The mammalian protein, siderocalin (Scn), binds siderophores and their ferric complexes as part of the innate immune system, and has also been shown to selectively bind a diverse range of Ln- and An-siderophore complexes. Scn is capable of specific, tight binding to a wide variety of metals complexes with natural and synthetic siderophores. In general, the binding of ligands/complexes in the protein calyx is driven by electrostatic and cation–π interactions, particularly by interactions between side chains and ligand aryl groups. Although perfected to accommodate hexadentate ligands like enterobactin in three pockets within the calyx, siderocalin manages to bind octadentate structures like HOPO by distorting the coordination environment of the calyx only mildly.

Crystals of the ternary LaIII–HOPO–Scn complex were also characterized for direct comparison between the +3 La/Ac metal centers. When compared to the structure of LaIII–HOPO–Scn that also crystallized in the P41212 space group with a resolution of 2.0 Å, the average La–OHOPO distance was 2.5(2) Å, which is nearly identical to the average La–OH2O bond length [2.55(5) Å] in the [LaIII(H2O)9]CF3SO3H solid-state structure. The most noteworthy structural rearrangement in the AcIII complex involves the movement of two aryl groups of the HOPO chelator, the one occupying Pocket #3 and the other extending out of the calyx, above another HOPO group, in Pocket #1 (red arrows). These movements displace the two aryl groups outwards, likely to accommodate the larger AcIII ion, and are not observed in the corresponding LaIII structure. We can speculate that the larger size of actinium (AcIII ionic radius = 1.065 A¨, CN = 6)28 enables closer interactions between the metal complex and key amino acids in the protein calyx, which are observed at longer distances in the lanthanum system (LaIII ionic radius = 1.032 A¨, CN = 6). For example, the two lysine residues (K125, K134) that define Pocket #1 have an average Ac···NζK125 distance of 4.0(4) Å vs. 4.5(1) Å for La···NζK125 and an average Ac···NζK134 distance of 3.9(1) Å vs. 4.5(1) Å for La···NζK134. Meanwhile, these results emphasize differences in the coordination behavior of lanthanum and actinium and collectively illustrate an example wherein the use of a non-radiological surrogate as a proxy for the radioactive ion did not fully capture their chemical complexities.

>[3x]QDSTSDLIPAPPLSKVPLQQNFQDNQFQGKWYVVGLAGNAILREDKDPQKMYATIYELKEDKSYNVTSVLFRKKKCDYWIRTFVPGSQPGEFTLGNIKSYPGLTSYLVRVVSTNYNQHAMVFFKKVSQNREYFKITLYGRTKELTSELKENFIRFSKSLGLPENHIVFPVPIDQCIDG Next, a β-keto acid cleavage enzyme (BKACE)28,29 converts the non-native substrate MSA with acetyl-CoA into acetoacetate and formyl-CoA. The Claisen-like condensation reaction accepts various β-keto acids that react with acetyl-CoA to form an acyl-CoA ester and acetoacetate. In these assays, BKACE15 from Paracoccus denitrificans performed best. BKACE15 forms a homotetramer where each active site is accommodated in a TIM-barrel fold, and consists of eight β-sheets that are surrounded by eight α-helices.

The two openings of the TIM barrel are closed off by smaller α-helices. As previously reported for the BKACE from Candidatus Cloacamonas acidaminovorans, a close homolog of BKACE15, each active site coordinates a single Zn2+ ion. We confirmed a 1:1 zinc binding ratio in BKACE15 using Inductively Coupled Plasma Optical Emission Spectroscopy (ICP-OES). The physiological role of this enzyme is unknown. However, the genetic context suggests that BKACE15 is involved in the degradation of aromatic compounds, while experimentally confirmed substrates include β-ketohexanoate, 3,5-dioxohexanoate, 5-hydroxy-β-ketohexanoate and β-ketopentanoate.

>[2x]MSLNGKVIITCAVTGAIHTPSMSPYLPVSASEITDAAIGAAEAGAAVIHLHARHEGDGSPDQSVEAFNPILGVIKQASDAVLNITTGGAPTMSIAERIQPAQHYRPELASLNMGTMNFGLFPMLNRYESQLKHQWERNYLGNKDIIFRNTFGDVEHVMTTLGAGGTRFEFECYDTSHLYNLKHFYDRGLVKGPLFIQTVFGLMGGIGAHPDDVLHMKRTADRLFGQDYRWSVLGAGRNQLNIAAMSAAMGGHVRVGLEDNLWAGKGRLAETNAQQVRAARQIVEGLGLEVATPAEARELLALKGGDQVNF>MGSSHHHHHHSSGLVPRGSHMASDKPADSGSSEVKELTVYVDEGYKSYIEEVAKAYEKEAGVKVTLKTGDALGGLDKLSLDNQNGNVPDVMMAPYDRVGSLGSDGQLSEVKLSDGAKTDDTTKSLVTAANGKVYGAPAVIESLVMYYNKDLVKDAPKTFADLENLAKDSKYAFAGEDGKTTAFLADWTNFYYTYGLLAGNGAYVFGQNGKDAKDIGLANDGSIVGINYAKSWYEKWPKGMQDTEGAGNLIQTQFQEGKTAAIIDGPWKAQAFKDAKVNYGVATIPTLPNGKEYAAFGGGKAWVIPQAVKNLEASQKFVDFLVATEQQKVLYDKTNEIPANTEARSYAEG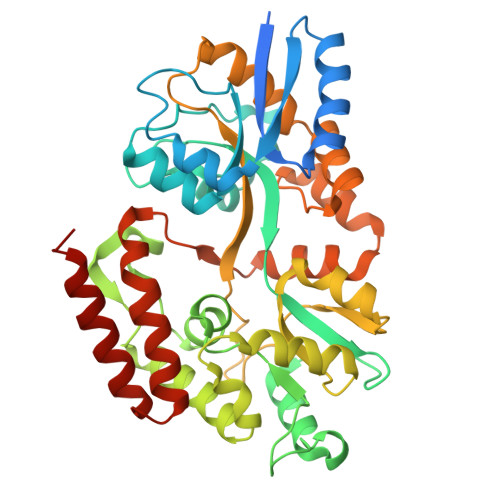KNDELTTAVIKQFKNTQPLPNISQMSAVWDPAKNMLFDAVSGQKDAKTAANDAVTLIKETLKQKFGE[2x]> QYAPQTQSGRTSIVHL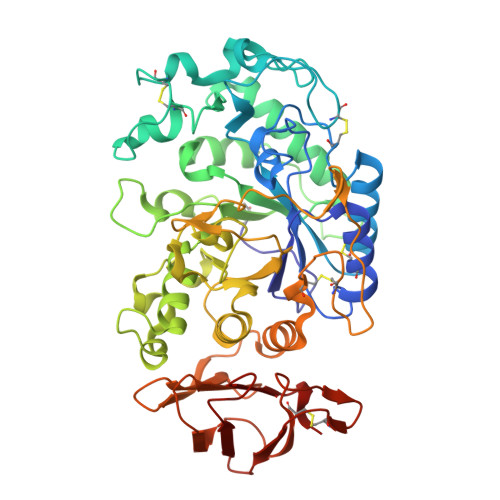FEWRWVDIALECERYLGPKGFGGVQVSPPNENVVVTNPSRPWWERYQPVSYKLCTRSGNENEFRDMVTRCNNVGVRIYVDAVINHMCGSGAAAGTGTTCGSYCNPGSREFPAVPYSAWDFNDGKCKTASGGIESYNDPYQVRDCQLVGLLDLALEKDYVRSMIADYLNKLIDIGVAGFRIDASKHMWPGDIKAVLDKLHNLNTNWFPAGSRPFIFQEVIDLGGEAISSSEYFGNGRVTEFKYGAKLGTVVRKWSGEKMSYLKNWGEGWGFMPSDRALVFVDNHDNQRGHGAGGSSILTFWDARLYKVAVGFMLAHPYGFTRVMSSYRWARNFVNGEDVNDWIGPPNNNGVIKEVTINADTTCGNDWVCEHRWREIRNMVWFRNVVDGQPFANWWDNGSNQVAFGRGNRGFIVFNNDDWQLSSTLQTGLPGGTYCNVISGDKVGNSCTGIKVYVSSDGTAQFSISNSAQDPFIAIHAESKL MaeK and MaeR exert their function by activating the expression of L-malate catabolic genes (maeP and maeE) and the expression of their own genes upon the presence of L-malate in the medium. Structural and phylogenetic analyses show that L. casei MaeKR proteins belong to the citrate family of TCS, as well as the characterized DcuSR and CitAB TCS. We also solved the crystal structure of the REC domain of MaeR in its activated state as well as the structure of a mutant version defective in the phosphoacceptor Asp. Altogether, our analysis has revealed that MaeKR is a non-canonical TCS conserved in Lactobacillales and that the structure of MaeR acknowledges the α4β5α5-swapped dimers as a new class of dimerization for RRs.

Crystals diffracted to 2.1 Å and the asymmetric unit contained two monomers of MaeRREC. The dimerization interface involves α4β5α5 structural elements, the main dimerization surface exploited by canonical RRs, such as the OmpR/PhoB family, but in MaeR β5 and α5 are swapped between subunits. This swapped conformation is due to a motion of the C-terminal β5α5 structural elements that swap from one monomer to the other by a rotation of about 178° (calculated by Dyndom33), using the loop β4-α4 and α4 as a hinge. To accomplish this swapping, α4 is reoriented and placed perpendicular to α3 instead of parallel, as is observed in the OmpR/PhoB family of RR. This motion allows the interaction of α4 from one subunit with α4 from the other subunit (α4*) and promotes new interactions that involve mainly β4 with β5* (and β4* with β5). Contrary to OmpR/PhoB dimers, where both active centres are placed in the same face of the dimer, they are located in opposite faces of the dimer in MaeR. The swapped MaeRREC dimer displays an interface area of about 2018 Å2 and a solvation free energy ∆iG of about −34 kcal.mol−1, suggesting that it is a tight dimer. The residues Thr82 and Tyr101, which correspond to the Y-T or aromatic switch, are oriented towards (inward) the active site. Interestingly, Lys104 and Tyr101, which contribute to the active site and to the Y-T switch respectively, are provided from swapped elements of the second monomer. In this way, the phosphorylated state cannot be reached unless the REC domain is swapped.

>MTNILIVEDDPMVQFIHRNYLEKIGTFDTIYSSETIADAKKLLASRSIQLVLLDIRLKDGNGIDFLTDLRRTKQTVDVILITAANEVNIVNDALHLGVIDYLIKPFTLERFEKSIQRYRTKH[2x]>MAEYVFSDAPKDSHGNGVKDAVPGKQPEELPPAPRYFQGENTAGFMRPVRFEGDITNLEVVGEIPKSIEGTFYRVMPEPHLPSFIPNDPWFNGDGNISGFYFKDGHVDLKQRYVRTEKFVREAEARRSLLGKYRNRYTDLVEFKIRSTANVNIVYWRGQLLALKEDSPPYAMDPETLETFGVYDFDGQLPSLTFTAHPKFDPVTREMVCFGYEAKGDGTRDICYYSFGPDGKIAETVWLVSPVCGMIHDFAVTENFVIFPIIPLVCDVERMKQGGDHWQWDYSIPMYIGVLPRRGAQGSDVKWFEAPHGFAGHVANAFEDDKGHIQLQMAYAKDNVFFWWPDANGKGPRPGEVEAHFANFVLDYQSDKLPLAEPTYLVDDDMEFPRIDDRVATRKHKHTFFCIFDRKPGVTDFEFVMPRAGGGAPMSNGLAHLNHETGDIQRYLPGPRKLTGECIFIPRNSEAAEGDGYVMVLLANYEDMCSELAVLDTKDLTNEVALIKLPVRLRPGLHGNWVDKSDVDGHPAPL[4x]

Carotenoid cleavage dioxygenases (CCDs) are non-heme FeII enzymes that catalyze the oxidative cleavage of alkene bonds in carotenoids, stilbenoids, and related compounds. pmcCarotenoid cleavage dioxygenases (CCDs) are a broadly distributed superfamily of enzymes that catalyze the reaction of dioxygen (O2) with carotenoids, stilbenoids, and related redox-active polyenes. These enzymes use a mononuclear non-heme FeII center to activate O2 for reaction with a specific alkene group in the substrate, generating carbonyl-containing products of importance in biological processes such as hormonal signaling and light detection. Unlike many mononuclear non-heme iron dioxygenases that coordinate their FeII centers using a 2-His, 1-Glu/Asp “facial triad” motif, CCDs use a 4-His cluster, three of which hydrogen bond to second-sphere carboxylates (Glu/Asp). While one coordination position is occupied by a solvent ligand as demonstrated by several crystallographic and spectroscopic investigations, the other is vacant because of apparent occlusion by a nearby methyl group of a semiconserved, second sphere residue (i.e., Thr/Val/Ile), making CCDs five-coordinate (5C) in their resting FeII states.

To further investigate the contribution of the occluding residue to the CAO1 active site structure, a T151V substitution was introduced at the occluding site, as found in some carotenoid-cleaving CCDs like NdCCD. As this decrease in energy reflects distortion toward trigonal bipyramidal geometry induced by substrate binding, the smaller magnitude of the shift indicates a more limited FeII geometric distortion. This difference in distortion was also manifested in the crystal structure of T151V FeII–CAO1 in complex with piceatannol where a ∼6° compression of ∠His197Nε–Fe–H2O is observed versus a 21° compression of the corresponding angle in the wildtype enzyme. Inspection of the piceatannol binding mode in the T151V structure revealed some small but notable differences compared with that of the wildtype enzyme that could be responsible for the different outcomes in iron center distortion. First, the β-ring of piceatannol is rotated ∼7° away from the Val151 side chain as expected based on the less favorable interaction between the piceatannol 3′-hydroxyl group and the non-native Val151 methyl group. As a possible consequence, the piceatannol molecule is shifted away from the iron center by ∼0.13 Å, which reduces steric interactions with the iron-bound solvent. This effect is enhanced by the shift of the iron away from the piceatannol binding site, thereby providing more space for the solvent to bind with less distortion away from planar geometry.>[4x]MKWEMGLQEEYIELIKAG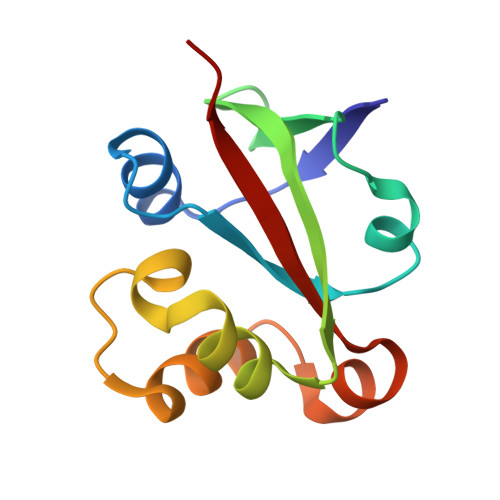KKKIEGRLYDEKRRQIKPGDIIIFEGGKLKVKVKGIRVYSSFKEMLEKEGIENVLPGVKSIEEGVKVYRQFYDEEREKKYGVVAIEIEPIE5-(2-aminopyrimidin-4-yl)-2-(5-chloro-2-methylphenyl)-1H-pyrrole-3-carboxamide | C16 H14 Cl N5 O | 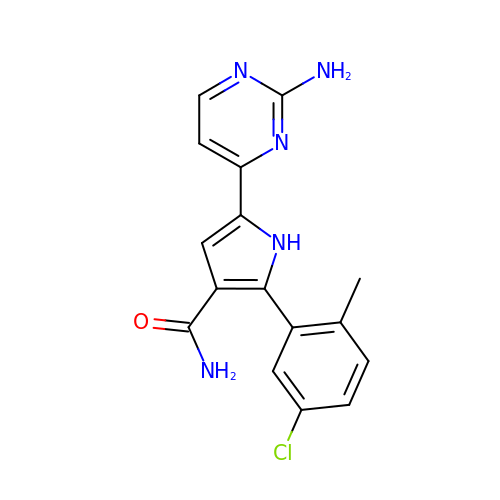DQDASFFHMDSYAZ-UHFFFAOYSA-N(1R)-1-methyl-1,2,3,4-tetrahydroisoquinoline | C10 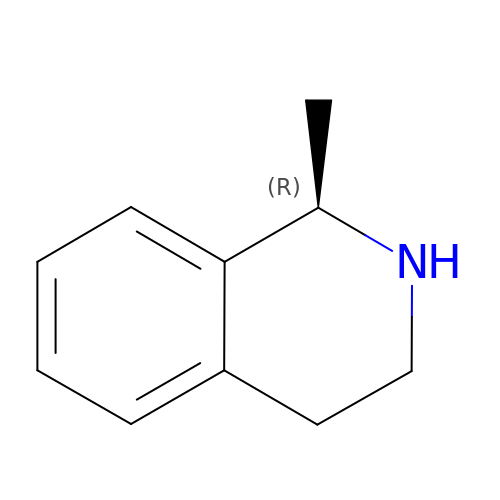H13 N | QPILYVQSKNWRDD-MRVPVSSYSA-N> GSHMDELYRQSLEII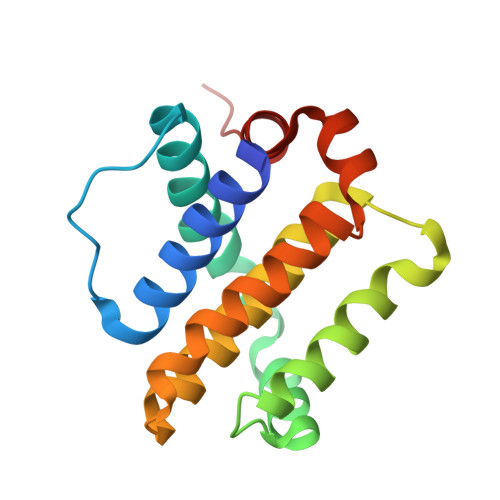SRYLREQATGAKDTKPMGRSGATSRKALETLRRVGDGVQRNHETAFQGMLRKLDIKNEDDVKSLSRVMIHVFSDGVTNWGRIVTLISFGAFVAKHLKTINQESCIEPLAESITDVLVRTKRDWLVKQRGWDGFVEFFHVED(3R,4S,5R)-5-[(1R)-1-CARBOXY-2,2-DIFLUORO-1-(PHOSPHONOOXY)ETHOXY]-4-HYDROXY-3-(PHOSPHONOOXY)CYCLOHEX-1-ENE-1-CARBOXYLIC 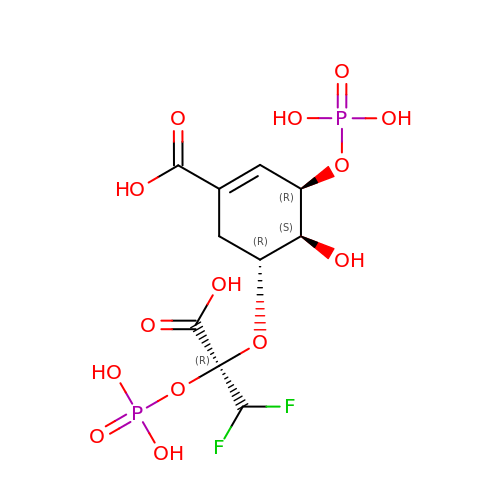ACID | C10 H14 F2 O14 P2 | OHXHNRRSMKIHDJ-VFWNUGQXSA-N>[2x]PPKLCLVCSDEASGCHYGVLT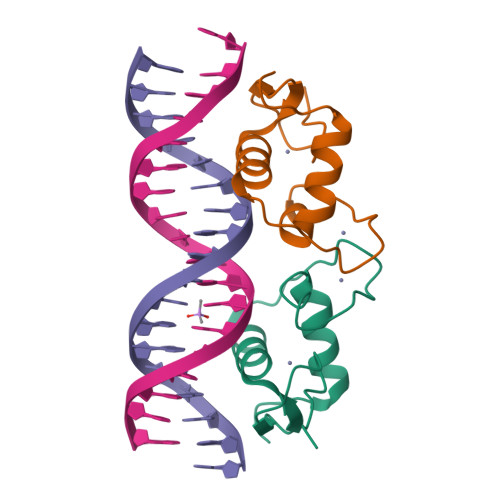CGSCKVFFKRAVEGQHNYLCAGRNDCIIDKIRRKNCPACRYRKCLQAGMNLEA Mitochondrial calcium uptake proteins 1 and 2 (MICU1 and MICU2) mediate mitochondrial Ca2+ influx via the mitochondrial calcium uniporter (MCU). Its molecular action for Ca2+ uptake is tightly controlled by the MICU1–MICU2 heterodimer, which comprises Ca2+ sensing proteins which act as gatekeepers at low [Ca2+] or facilitators at high [Ca2+]. Intriguingly, humans have three MICU paralogs (MICU1, MICU2 and MICU3), as well as an alternative splicing variant (MICU1.1) depending on the tissues, and human MICU1 and MICU2 generally assemble as a heterodimer and regulate Ca2+ uptake of the MCU complex in most tissues. In particular, it has been reported that MICU2 functions as a gatekeeper of the MCU for suppressing the cellular damage caused by excessive mitochondrial Ca2+ influx.

Four MICU1–MICU2 heterodimers were observed per asymmetric unit (ASU). The heterodimers were formed by a face-to-face (F–F) interface similar to other MICU homodimer structures [Figs. 1(a) and 1(b)]. Unlike MICU homodimer structures, the MICU1–MICU2 heterodimer comprised two interfaces, interfaces 1 and 2, as a result of the asymmetry of the heterodimer. Therefore, the interfaces of the MICU1–MICU2 heterodimer contained a rigid interface 1 and a variable interface 2. Compared with the homodimers in MICU1 and MICU2, only structural differences in the interloop (L6) of MICU1 EF-hand 1 were observed in interface 1 comprising MICU1 EF-hand 1 and MICU2 EF-hand 3. The primary interactions between MICU1 and MICU2 were two salt bridges involving the highly conserved side chains of Arg221(MICU1)–Asp330(MICU2) and Asp231(MICU1)–Arg352(MICU2) [Figs. 3(a), S4 and S5]. In contrast, the other salt bridge, Asp231(MICU1)–Arg352(MICU2), has never been observed in other MICU homodimer structures. Notably, the Asp231(MICU1) was located on the interloop (L6) of EF-hand 1 participating in the Ca2+ coordination, indicating that Ca2+ binding induces structural changes directly on interface 1. The tight interaction in the apo state of MICU1–MICU2 might hinder the conformational changes required for Ca2+ binding, resulting in a lower Ca2+ binding affinity in the MICU1–MICU2 heterodimer compared with that of the MICU1 homodimer.

>[4x]EEKKKKRSGFRDRKVMEYENRIRAYSTPDKIFRYFATLKVISEPGEAEVFMTPEDFVRSITPNEKQPEHLGLDQYIIKRFDGKKISQEREKFADEGSIFYTLGECGLISFSDYIFLTTVLSTPQRNFEIAFKMFDLNGDGEVDMEEFEQVQSIIRSQTSMGMRHRDRPTTGNTLKSGLCSALTTYFFGADLKGKLTIKNFLEFQRKLQHDVLKLEFERHDPVDGRITERQFGGMLLAYSGVQSKKLTAMQRQLKKHFKEGKGLTFQEVENFFTFLKNINDVDTALSFYHMAGASLDKVTMQQVARTVAKVELSDHVCDVVFALFDCDGNGELSNKEFVSIMKQRLMRG;>HHHHHHMSLRKQRFMQFSSLEHEGEYYMTPRDFLFSVMFEQMERKTSVKKLTKKDIEDTLSGIQTAGCGSTFFRDLGDKGLISYTEYLFLLTILTKPHSGFHVAFKMLDTDGNEMIEKREFFKLQKIISKQDDLMTVKTNETGYQEAIVKEPEINTTLQMRFFGKRGQRKLHYKEFRRFMENLQTEIQEMEFLQFSKGLSFMRKEDFAEWLLFFTNTENKDIYWKNVREKLSAGESISLDEFKSFCHFTTHLEDFAIAMQMFSLAHRPVRLAEFKRAVKVATGQELSNNILDTVFKIFDLDGDECLSHEEFLGVLKNRMHRGLWV[4x]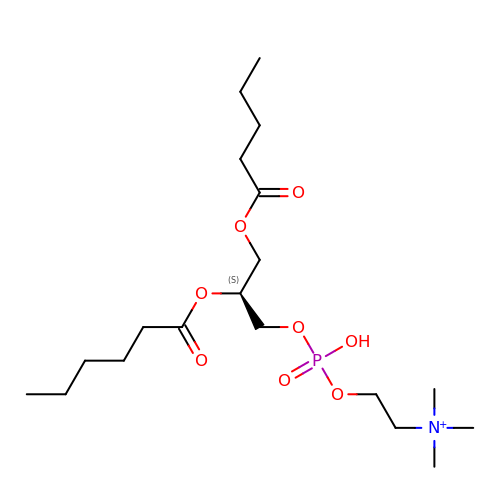(4R,7S)-4-hydroxy-N,N,N-trimethyl-4,9-dioxo-7-[(pentanoyloxy)methyl]-3,5,8-trioxa-4lambda~5~-phosphatetradecan-1-aminium | C19 H39 N O8 P | IZTOQGOABQJQQN-KRWDZBQOSA-O> MWISIKTLIHHLGVLFFCDYMYNRREKKIIEVKTMRITKVEVDRKKVLISRDKNGGKLVYENEMQDNTEQIMHHKKSSFYKSVVNKTICRPEQKQMKKLVHGLLQENSQEKIKVSDVTKLNISNFLNHRFKKSLYYFPENSPDKSEEYRIEINLSQLLEDSLKKQQGTFICWESFSKDMELYINWAENYISSKTKLIKKSIRNNRIQSTESRSGQLMDRYMKDILNKNKPFDIQSVSEKYQLEKLTSALKATFKEAKKNDKEINYKLKSTLQNHERQIIEELKENSELNQFNIEIRKHLETYFPIKKTNRKVGDIRNLEIGEIQKIVNHRLKNKIVQRILQEGKLASYEIESTVNSNSLQKIKIEEAFALKFINACLFASNNLRNMVYPVCKKDILMIGEFKNSFKEIKHKKFIRQWSQFFSQEITVDDIELASWGLRGAIAPIRNEIIHLKKHSWKKFFNNPTFKVKKSKIINGKTKDVTSEFLYKETLFKDYFYSELDSVPELIINKMESSKILDYYSSDQLNQVFTIPNFELSLLTSAVPFAPSFKRVYLKGFDYQNQDEAQPDYNLKLNIYNEKAFNSEAFQAQYSLFKMVYYQVFLPQFTTNNDLFKSSVDFILTLNKERKGYAKAFQDIRKMNKDEKPSEYMSYIQSQLMLYQKKQEEKEKINHFEKFINQVFIKGFNSFIEKNRLTYICHPTKNTVPENDNIEIPFHTDMDDSNIAFWLMCKLLDAKQLSELRNEMIKFSCSLQSTEEISTFTKAREVIGLALLNGEKGCNDWKELFDDKEAWKKNMSLYVSEELLQSLPYTQEDGQTPVINRSIDLVKKYGTETILEKLFSSSDDYKVSAKDIAKL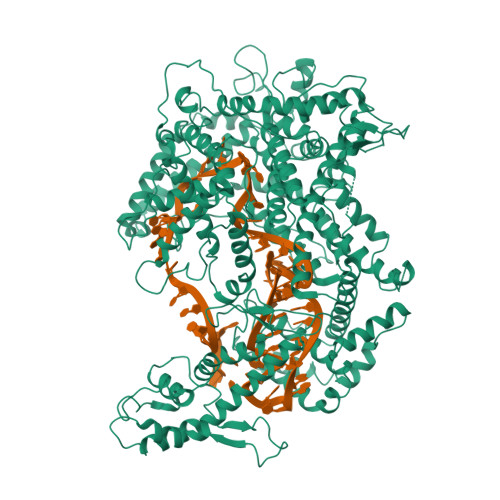HEYDVTEKIAQQESLHKQWIEKPGLARDSAWTKKYQNVINDISNYQWAKTKVELTQVRHLHQLTIDLLSRLAGYMSIADRDFQFSSNYILERENSEYRVTSWILLSENKNKNKYNDYELYNLKNASIKVSSKNDPQLKVDLKQLRLTLEYLELFDNRLKEKRNNISHFNYLNGQLGNSILELFDDARDVLSYDRKLKNAVSKSLKEILSSHGMEVTFKPLYQTNHHLKIDKLQPKKIHHLGEKSTVSSNQVSNEYCQLVRTLLTMKHHHHHH> AAQTNAPWGLARISSTSPGTSTYYYDESAGQGSCVYVIDTGIEASHPEFEGRAQMVKTYYYSSRDGNGHGTHCAGTVGSRTYGVVKKTQLFGVKVLDDNGS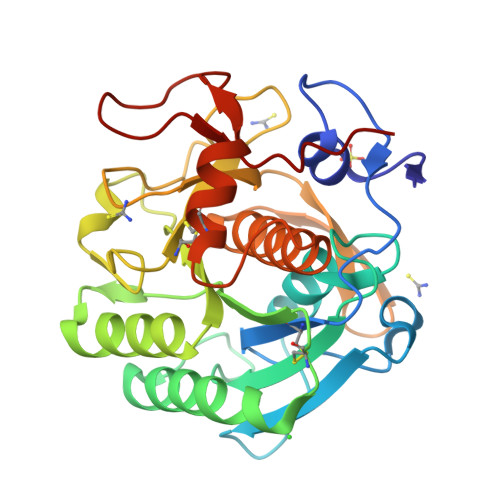GQYSTIIAGMDFVASDKNNRNCPKGVVASLSLGGGYSSSVNSAAARLQSSGVMVAVAAGNNNADARNYSPASEPSVCTVGASDRYDRRSSFSNYGSVLDIFGPGTSILSTWIGGSTRSISGTSMATPHVAGLAAYLMTLGKTTAASACRYIADTANKGDLSNIPFGTVNLLAYNNYQA7-PYRIDIN-2-YL-N-(3,4,5-TRIMETHOXYPHENYL)-7H-PYRROLO[2,3-D]PYRIMIDIN-2-AMINE | C20 H19 N5 O3 | 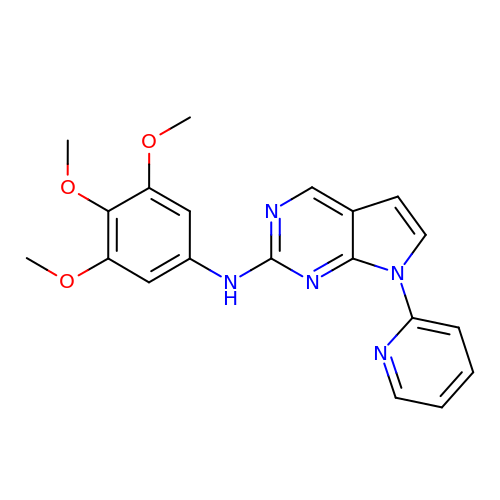YENZSPIOXMNEFF-UHFFFAOYSA-N>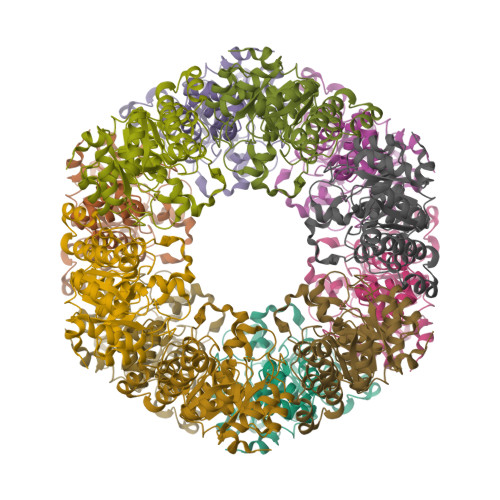[12x]HGTELIKRGFARMQKGGVIMDVTTPEQARIAEEAGAVAVMALQAVPADIRKAGGVARMADPEIVQQIIETVTIPVMAKARIGHFVEAEILEALGVDMVDESEVLTPADPFYHIDKTQFTVPFVCGARNLGEALRRINEGAAMIRTKGEAGTGDVSQAVKHMKQIQGEIRALAGKTKEELIMVAREIEAPIELVVETAKMQRLPVVNFAAGGVATPADAALMMRLGADGVFVGSGIFKAENPEKMAKAVVEAVNNYDNPVKLAEISKGVGAGMKGISADMIPAQEALQERGW>GPLGSMTNKELQAIRKLLMLDVSEAAEHIGRVSARSWQYWESGRSAVPDDVEQEMLDLASVRI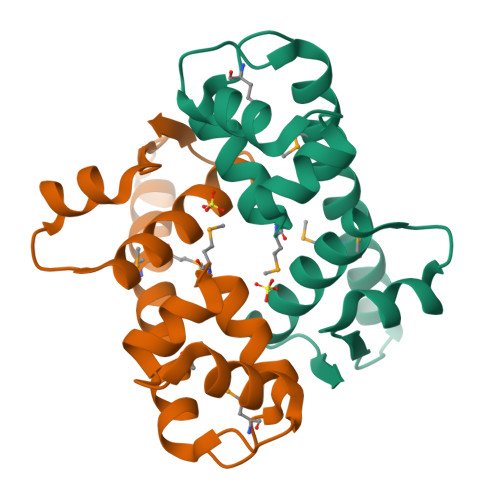EMMSAIDKRLADGERPKLRFYNKLDEYLADNPDHNVIGWRLSQSVAALYYTEGHADLI[2x]> MKLDIKKTFSNRSDRVKGIDFHPTEPWVLTTLYSG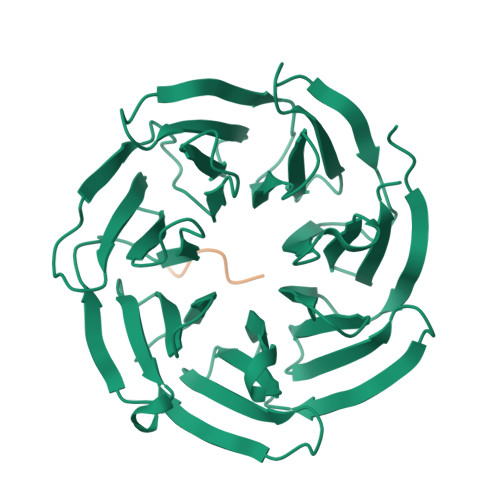RVEIWNYETQVEVRSIQVTETPVRAGKFIARKNWIIVGSDDFRIRVFNYNTGEKVVDFEAHPDYIRSIAVHPTKPYVLSGSDDLTVKLWNWENNWALEQTFEGHEHFVMCVAFNPKDPSTFASGCLDRTVKVWSLGQSTPNFTLTTGQERGVNYVDYYPLPDKPYMITASDDLTIKIWDYQTKSCVATLEGHMSNVSFAVFHPTLPIIISGSEDGTLKIWNSSTYKVEKTLNVGLERSWCIATHPTGRKNYIASGFDNGFTVLSLA;> EKVHVQ[(2~{R},3~{R})-2,3-bis(oxidanyl)-3-[[(2~{S})-3-oxidanylidenepent-4-en-2-yl]amino]propyl] dihydrogen phosphate | C8 H16 N O7 P | 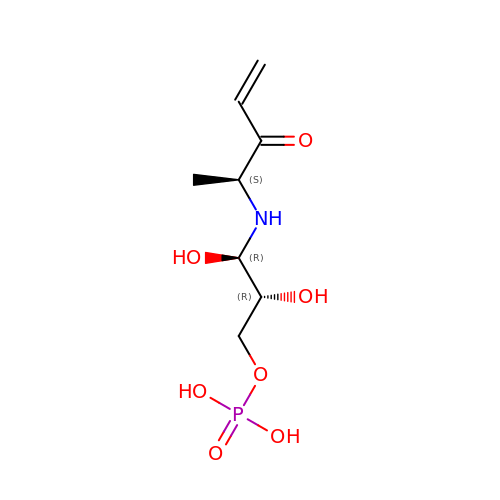UJGBYPNOGNUCKJ-UIISKDMLSA-N> MGSDKIHHHHHHMKIDILDKGFVELVDVMGNDLSAVRA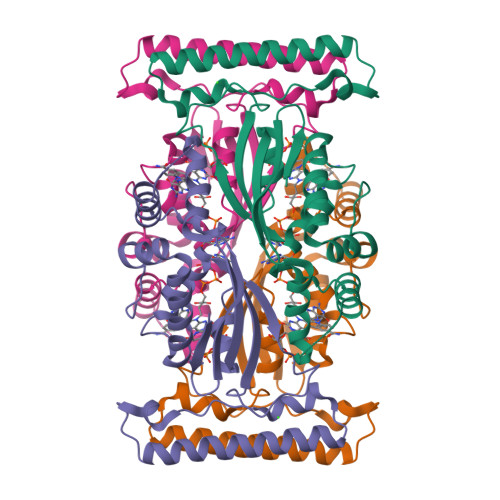ARVSFDMGLKDEERDRHLIEYLMKHGAETPFEHIVFTFHVKAPIFVARQWFRHRIASYNELSGRYSKLSYEFYIPSPERLEGYKTTIPPERVTEKISEIVDKAYRTYLELIESGVPREVARIVLPLNLYTRFFWTVNARSLMNFLNLRADSHAQWEIQQYALAIARIFKEKCPWTFEAFLKYAYKGDILKEVQV>GSMEPAMEPETLEARINRATNPLNKELDWASINGFCEQLN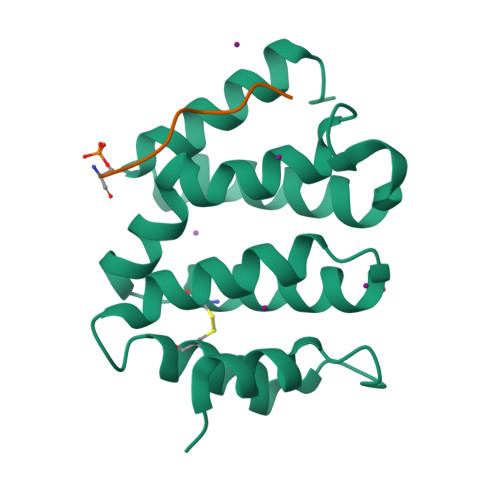EDFEGPPLATRLLAHKIQSPQEWEAIQALTVLETCMKSCGKRFHDEVGKFRFLNELIKVVSPKYLGSRTSEKVKNKILELLYSWTVGLPEEVKIAEAYQMLKKQGIVKS[2x];>[2x]ITGFSDDVPMVIA> SLQMVTVGHNIALIQPGFSLMNFDGQVFFFGQKGWPKRSCPTGVFHFDIKQNHLKLKPAIFSKDSCYLPPLRYPATCSYKGSIDSDKHQYIIHGGKTPNNELSDKIYIMSVACKNNKKVTFRCTEKDLVGDVPEPRYGHSIDVVYSRGKSMGVLFGGRSYMPSTQRTTEKWNSVADCLPHVFLIDFEFGCATSYILPELQDGLSFHVSIARNDTVYILGGHSLASNIRPANLYRIRVDLPLGTPAVNCTVLPGGISVSSAILTQTNNDEFVIVGGYQLENQKRM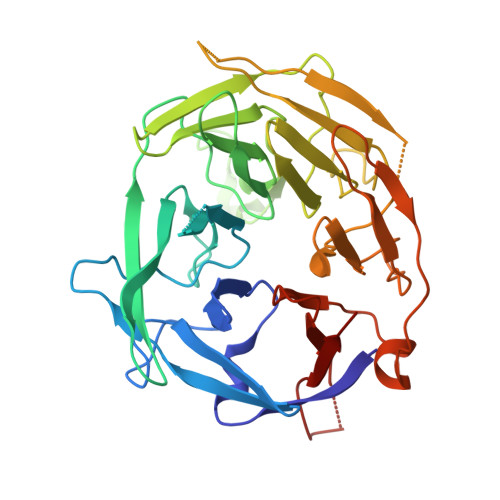VCSLVSLGDNTIEISEMETPDWTSDIKHSKIWFGSNMGNGTIFLGIPGDNKQAMSEAFYFYTLRC>MGREKTLCKSWSDMKKHLNDTVSKSFIGRFFKLEARKTTFTTELRAATATFLTMAYIITVNANILADSGATCSINDCSTVASSSPPGPECVLGSNPGYEQCISRVKKDLVVATSLSAMVGSLAMGLLANLPFGLAPGMGANAYIAYNVVGFRGSGS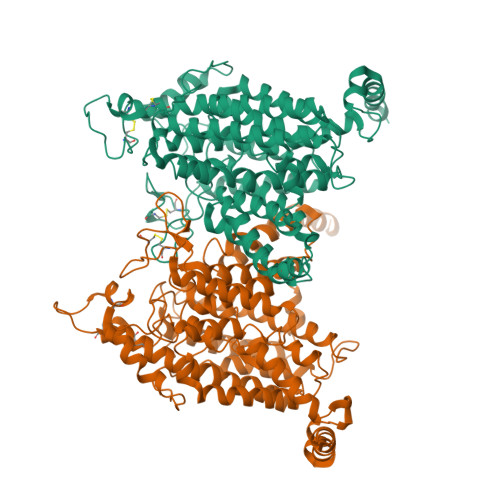ISYHTAMAIVLLEGCAFLAVSALGLRGKLARLIPQTVRLACAVGIGMFIAFVGLQMNQGIGLVGPDKSTLVTLTACAETDPVTGACLGGKMKSPTFWLAVVGFLITSFGLMKNVKGSMIYGIVFVTAISWIRGTQVTIFPHTPLGDSNYNYFTKIVDFHKIQSTLGAISFTEFRKSEVWVAFATLFYVDLLGTTGVLYTMAEIGGFVEDGKFEGEYAAYLVDAGSSVVGSALGVTTTATFVESSAGLKEGGKTGLTAVIVGLYFLASMFFTPLVTNVPRWAVGPSLVMVGVMMMGVVKDIRWGETKEAVTAFVTILLMPLTYSIANGIIAGIGIYLALSMYDVVLGVAKWLNGVRKRVMREHNQVSSVATVEIV[2x]> MNAYQNDKLHLCAPRPDLVRAAM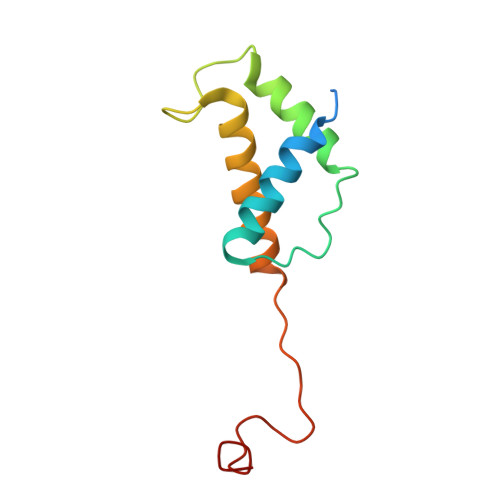SAMVRETGCTPNVNIREMAISAGVMLTKIRANPGMLRYGMTATQTVIYNLKELFAAHAARGVVFKTPAIHPAHPSQWKGF> SSLLEKGLDGAKKAVGG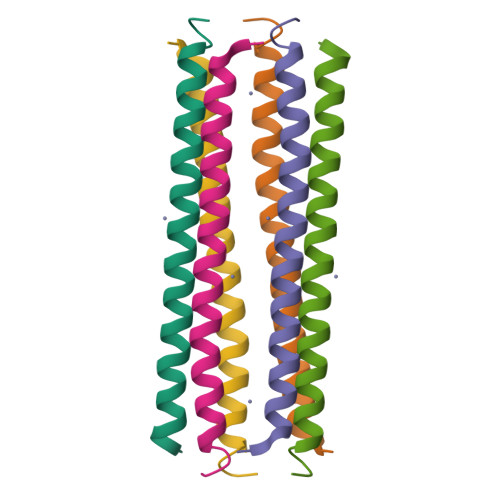LGKLGKDAVEDLESVGKGAVHDVKDVLDSVL> MFDTKLFLSLPIDIRYTVYFFLGDVVQNVRPPAKSDIFNDELIAYPNIREFNQSLVDKYSKHIGVYDYIPNFIPNWCRDFDLLRHDIILTDRLRVCLQYEEQWFSVQWIVVSGELEIGIFTTDEQFLQVSYTINEYCHLLSIAQQDLRLGINVSDINDVNELCKEIQHRWLFDTVSYISFINCWDLDHENVVSIIPCMESFNNLHMLRIESKNMFNNLINTQGVRENPGKTIVYNVRQNIFELELYTLRDLGYKSVVDLQKWEQLQCLSLSGCEFIDLNNLIL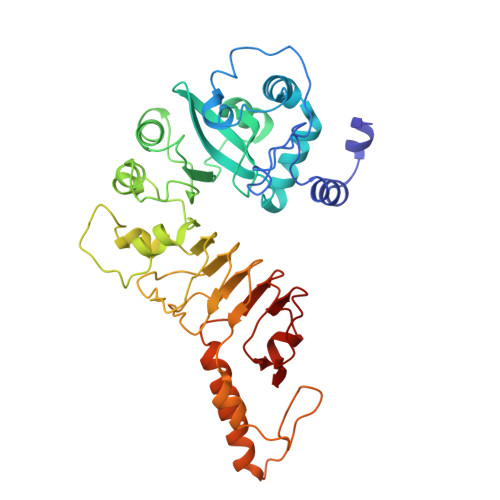PQHCKMLILKEVKYIIWWDLSHLLKRIRPQWIINGQVKKPTKKEEEEESEWYNLYLEVVQTYQPLNFIELHNAKRVKGNLILPARLVTESRIKISNGTKVDSVLLI Type I fungal FAS forms a barrel-shaped complex composed of two reaction chambers. Six β-chains form the walls of the barrel while a central wheel, made by the six α-chains, bisects the barrel into two chemically identical reaction chambers. Therefore, each chamber has three complete sets of catalytic domains including three acyl-carrier protein (ACP) domains. Substrates are shuttled between the static reaction centers by the mobile ACP domain flexibly tethered at its N and C termini.

We used cryoEM to reconstruct ab initio ACP densities inside the reaction chambers of endogenous fungal FASs from S. cerevisiae and the opportunistic pathogen Candida albicans in the Apo and KS-stalled state, at 12 Å resolution, allowing localization of densities corresponding to this mobile domain. In the Apo state, ACP density is strongest in proximity of the KS domain in S. cerevisiae FAS and allows for a complete tracing of its backbone atoms in the high resolution cryoEM map. Examining the surface electrostatics of ACP- KS- and ER-domains shows a strong surface charge complementarity between the structural lobe of ACP with the KS domain in S. cerevisiae. In S. cerevisiae FAS, second strongest ACP density is observed at lower resolution and less stringent threshold of the AAI map that shows ACP near the apical region of the reaction chamber and facing the AT catalytic site. In both FASs in the Apo state, the structural lobe of ACP has stronger and better resolved densities compared to the canonical lobe in the KS-binding site, as observed in the high-resolution refined maps, suggesting a more stable interaction between the former and the KS-domain in the absence of substrates. Interestingly, in the S. cerevisiae Apo and KS-stalled states, where no ACP density can be seen by the ER domain, the catalytic histidine side chain is in a single conformation facing FMN.

> MKPEVEQELAHILLTELLAYQFASPVRWIETQDVFLKDFNTERVVEIGPSPTLAGMAQRTLKNKYESYDAALSLHREILCYSKDAKEIYYTPDPSELAAKEEPAKEEAPAPTPAANAPAPAAAAPAPVAAAAPAAAAAEIADEPVKASLLLHVLVAHKLKKSLDSIPMSKTIKDLVGGKSTVQNEILGDLGKEFGTTPEKPEETPLEELAETFQDTFSGALGKQSSSLLSRLISSKMPGGFTITVARKYLQTRWGLPSGRQDGVLLVALSNEPAARLGSEADAKAFLDSMAQKYASIVGVDLSSAASASGAAGAGAAAGAAMIDAGALEEITKDHKVLARQQLQVLARYLKMDLDNGERKFLKEKDTVAELQAQLDYLNAELGEFFVNGVATSFSRKKARTFDSSWNWAKQSLLSLYFEIIHGVLKNVDREVVSEAINIMNRSNDALIKFMEYHISNTDETKGENYQLVKTLGEQLIENCKQVLDVDPVYKDVAKPTGPKTAIDKNGNITYSEEPREKVRKLSQYVQEMALGGPITKESQPTIEEDLTRVYKAISAQADKQDISSSTRVEFEKLYSDLMKFLESSKEIDPSQTTQLAGMDVEDALDKDSTKEVASLPNKSTISKTVSSTIPRETIPFLHLRKKTPAGDWKYDRQLSSLFLDGLEKAAFNGVTFKDKYVLITGAGKGSIGAEVLQGLLQGGAKVVVTTSRFSKQVTDYYQSIYAKYGAKGSTLIVVPFNQGSKQDVEALIEFIYDTEKNGGLGWDLDAIIPFAAIPEQGIELEHIDSKSEFAHRIMLTNILRMMGCVKKQKSARGIETRPAQVILPMSPNHGTFGGDGMYSESKLSLETLFNRWHSESWANQLTVCGAIIGWTRGTGLMSANNIIAEGIEKMGVRTFSQKEMAFNLLGLLTPEVVELCQKSPVMADLNGGLQFVPELKEFTAKLRKELVETSEVRKAVSIETALEHKVVNGNSADAAYAQVEIQPRANIQLDFPELKPYKQVKQIAPAELEGLLDLERVIVVTGFAEVGPWGSARTRWEMEAFGEFSLEGCVEMAWIMGFISYHNGNLKGRPYTGWVDSKTKEPVDDKDVKAKYETSILEHSGIRLIEPELFNGYNPEKKEMIQEVIVEEDLEPFEASKETAEQFKHQHGDKVDIFEIPETGEYSVKLLKGATLYIPKALRFDRLVAGQIPTGWNAKTYGISDDIISQVDPITLFVLVSVVEAFIASGITDPYEMYKYVHVSEVGNCSGSGMGGVSALRGMFKDRFKDEPVQNDILQESFINTMSAWVNMLLISSSGPIKTPVGACATSVESVDIGVETILSGKARICIVGGYDDFQEEGSFEFGNMKATSNTLEEFEHGRTPAEMSRPATTTRNGFMEAQGAGIQIIMQADLALKMGVPIYGIVAMAATATDKIGRSVPAPGKGILTTAREHHSSVKYASPNLNMKYRKRQLVTREAQIKDWVENELEALKLEAEEIPSEDQNEFLLERTREIHNEAESQLRAAQQQWGNDFYKRDPRIAPLRGALATYGLTIDDLGVASFHGTSTKANDKNESATINEMMKHLGRSEGNPVIGVFQKFLTGHPKGAAGAWMMNGALQILNSGIIPGNRNADNVDKILEQFEYVLYPSKTLKTDGVRAVSITSFGFGQKGGQAIVVHPDYLYGAITEDRYNEYVAKVSAREKSAYKFFHNGMIYNKLFVSKEHAPYTDELEEDVYLDPLARVSKDKKSGSLTFNSKNIQSKDSYINANTIETAKMIENMTKEKVSNGGVGVDVELITSINVENDTFIERNFTPQEIEYCSAQPSVQSSFAGTWSAKEAVFKSLGVKSLGGGAALKDIEIVRVNKNAPAVELHGNAKKAAEEAGVTDVKVSISHDDLQAVAVAVSTKK;> MDAYSTRPLTLSHGSLEHVLLVPTASFFIASQLQEQFNKILPEPTEGFAADDEPTTPAELVGKFLGYVSSLVEPSKVGQFDQVLNLCLTEFENCYLEGNDIHALAAKLLQENDTTLVKTKELIKNYITARIMAKRPFDKKSNSALFRAVGEGNAQLVAIFGGQGNTDDYFEELRDLYQTYHVLVGDLIKFSAETLSELIRTTLDAEKVFTQGLNILEWLENPSNTPDKDYLLSIPISCPLIGVIQLAHYVVTAKLLGFTPGELRSYLKGATGHSQGLVTAVAIAETDSWESFFVSVRKAITVLFFIGVRCYEAYPNTSLPPSILEDSLENNEGVPSPMLSISNLTQEQVQDYVNKTNSHLPAGKQVEISLVNGAKNLVVSGPPQSLYGLNLTLRKAKAPSGLDQSRIPFSERKLKFSNRFLPVASPFHSHLLVPASDLINKDLVKNNVSFNAKDIQIPVYDTFDGSDLRVLSGSISERIVDCIIRLPVKWETTTQFKATHILDFGPGGASGLGVLTHRNKDGTGVRVIVAGTLDINPDDDYGFKQEIFDVTSNGLKKNPNWLEEYHPKLIKNKSGKIFVETKFSKLIGRPPLLVPGMTPCTVSPDFVAATTNAGYTIELAGGGYFSAAGMTAAIDSVVSQIEKGSTFGINLIYVNPFMLQWGIPLIKELRSKGYPIQFLTIGAGVPSLEVASEYIETLGLKYLGLKPGSIDAISQVINIAKAHPNFPIALQWTGGRGGGHHSFEDAHTPMLQMYSKIRRHPNIMLIFGSGFGSADDTYPYLTGEWSTKFDYPPMPFDGFLFGSRVMIAKEVKTSPDAKKCIAACTGVPDDKWEQTYKKPTGGIVTVRSEMGEPIHKIATRGVMLWKEFDETIFNLPKNKLVPTLEAKRDYIISRLNADFQKPWFATVNGQARDLATMTYEEVAKRLVELMFIRSTNSWFDVTWRTFTGDFLRRVEERFTKSKTLSLIQSYSLLDKPDEAIEKVFNAYPAAREQFLNAQDIDHFLSMCQNPMQKPVPFVPVLDRRFEIFFKKDSLWQSEHLEAVVDQDVQRTCILHGPVAAQFTKVIDEPIKSIMDGIHDGHIKKLLHQYYGDDESKIPAVEYFGGESPVDVQSQVDSSSVSEDSAVFKATSSTDEESWFKALAGSEINWRHASFLCSFITQDKMFVSNPIRKVFKPSQGMVVEISNGNTSSKTVVTLSEPVQGELKPTVILKLLKENIIQMEMIENRTMDGKPVSLPLLYNFNPDNGFAPISEVMEDRNQRIKEMYWKLWIDEPFNLDFDPRDVIKGKDFEITAKEVYDFTHAVGNNCEDFVSRPDRTMLAPMDFAIVVGWRAIIKAIFPNTVDGDLLKLVHLSNGYKMIPGAKPLQVGDVVSTTAVIESVVNQPTGKIVDVVGTLSRNGKPVMEVTSSFFYRGNYTDFENTFQKTVEPVYQMHIKTSKDIAVLRSKEWFQLDDEDFDLLNKTLTFETETEVTFKNANIFSSVKCFGPIKVELPTKETVEIGIVDYEAGASHGNPVVDFLKRNGSTLEQKVNLENPIPIAVLDSYTPSTNEPYARVSGDLNPIHVSRHFASYANLPGTITHGMFSSASVRALIENWAADSVSSRVRGYTCQFVDMVLPNTALKTSIQHVGMINGRKLIKFETRNEDDVVVLTGEAEIEQPVTTFVFTGQGSQEQGMGMDLYKTSKAAQDVWNRADNHFKDTYGFSILDIVINNPVNLTIHFGGEKGKRIRENYSAMIFETIVDGKLKTEKIFKEINEHSTSYTFRSEKGLLSATQFTQPALTLMEKAAFEDLKSKGLIPADATFAGHSLGEYAALASLADVMSIESLVEVVFYRGMTMQVAVPRDELGRSNYGMIAINPGRVAASFSQEALQYVVERVGKRTGWLVEIVNYNVENQQYVAAGDLRALDTVTNVLNFIKLQKIDIIELQKSLSLEEVEGHLFEIIDEASKKSAVKPRPLKLERGFACIPLVGISVPFHSTYLMNGVKPFKSFLKKNIIKENVKVARLAGKYIPNLTAKPFQVTKEYFQDVYDLTGSEPIKEIIDNWEKYEQSDYKDHDGDYKDHDIDYKDDDDK> MAKDIEISASESKFILEALRQNYRLDGRSFDQFRDVEITFGKEFGDVSVKMGNTKVHCRISCQIAQPYEDRPFEGLFVISTEISPMAGSQFENGNITGEDEVLCSRIIEKSVRRSGALDVEGLCIVAGSKCWAVRADVHFLDCDGGFIDASCIAVMAGLMHFKKPDITVHGEQIIVHPVNEREPVPLGILHIPICVTFSFFNPQDTEENIKGETNSEISIIDATLKEELLRDGVLTVTLNKNREVVQVSKAGGLPMDALTLMKCCHEAYSIIEKITDQILQLLKEDSEKRNKYAAMLTSENAREI;> GPDHMSRLEIYSPEGLRLDGRRWNELRRFESSINTHPHAADGSSYMEQGNNKIITLVKGPKEPRLKSQMDTSKALLNVSVNITKFSKFERSKSSHKNERRVLEIQTSLVRMFEKNVMLNIYPRTVIDIEIHVLEQDGGIMGSLINGITLALIDAGISMFDYISGISVGLYDTTPLLDTNSLEENAMSTVTLGVVGKSEKLSLLLVEDKIPLDRLENVLAIGIAGAHRVRDLMDEELRKHAQKRVSNASAR;> MAESTTLETIEIHPITFPPEVLARISPELSLQRHLSLGIRPCLRKYEEFRDVAIENNTLSRYADAGNIDTKNNILGSNVLKSGKTIVITSITGGIIEETSAAIKDLDDFGEEELFEVTKEEDIIANYASVYPVVEVERGRVGACTDEEMTISQKLHDSILHSRILPKKALKVKAGVRSANEDGTFSVLYPDELEDDTLNETNLKMKRKWSYVLYAKIVVLSRTGPVFDLCWNSLMYALQSVKLPRAFIDERASDLRMTIRTRGRSATIRETYEIICDQTKSVPLMINAKNIAFASNYGIVELDPECQLQNSDNSEEEEVDIDMDKLNTVLIADLDTEAEETSIHSTISILAAPSGNYKQLTLVGGGAKITPEMIKRSLLLSRVRADDLSTRFNI;> GSMSVQAEIGILDHVDGSSEFVSQDTKVICSVTGPIEPKARQELPTQLALEIIVRPAKGVATTREKVLEDKLRAVLTPLITRHCYPRQLCQITCQILESGEDEAEFSLRELSCCINAAFLALVDAGIALNSMCASIPIAIIKDTSDIIVDPTAEQLKISLSVHTLALEFVNGGKVVKNVLLLDSNGDFNEDQLFSLLELGEQKCQELVTNIRRIIQDNISPRLVV;> GDPHMSLSVAEKSYLYDSLASTPSIRPDGRLPHQFRPIEIFTDFLPSSNGSSRIIASDGSECIVSIKSKVVDHHVENELLQVDVDIAGQRDDALVVETITSLLNKVLKSGSGVDSSKLQLTKKYSFKIFVDVLVISSHSHPVSLISFAIYSALNSTYLPKLISAFDDLEVEELPTFHDYDMVKLDINPPLVFILAVVGNNMLLDPAANESEVANNGLIISWSNGKITSPIRSVALNDSNVKSFKPHLLKQGLAMVEKYAPDVVRSLENL;> MNVQDRRRLLGPAAAKPMAFSNTTTHVPEKKSTDLTPKGNESEQELSLHTGFIENCNGSALVEARSLGHQTSLITAVYGPRSIRGSFTSQGTISIQLKNGLLEKYNTNELKEVSSFLMGIFNSVVNLSRYPKSGIDIFVYLTYDKDLTNNPQDDDSQSKMMSSQISSLIPHCITSITLALADAGIELVDMAGAGEANGTVVSFIKNGEEIVGFWKDDGDDEDLLECLDRCKEQYNRYRDLMISCLMNQET;> GDPHMSTFIFPGDSFPVDPTTPVKLGPGIYCDPNTQEIRPVNTGVLHVSAKGKSGVQTAYIDYSSKRYIPSVNDFVIGVIIGTFSDSYKVSLQNFSSSVSLSYMAFPNASKKNRPTLQVGDLVYARVCTAEKELEAEIECFDSTTGRDAGFGILEDGMIIDVNLNFARQLLFNNDFPLLKVLAAHTKFEVAIGLNGKIWVKCEELSNTLACYRTIMECCQKNDTAAFKDIAKRQFKEILTVKEE;> GDPHMSEVITITKRNGAFQNSSNLSYNNTGISDDENDEEDIYMHDVNSASKSESDSQIVTPGELVTDDPIWMRGHGTYFLDNMTYSSVAGTVSRVNRLLSVIPLKGRYAPETGDHVVGRIAEVGNKRWKVDIGGKQHAVLMLGSVNLPGGILRRKSESDELQMRSFLKEGDLLNAEVQSLFQDGSASLHTRSLKYGKLRNGMFCQVPSSLIVRAKNHTHNLPGNITVVLGVNGYIWLRKTSQMDLARDTPSANNSSSIKSTGPTGAVSLNPSITRLEEESSWQIYSDENDPSISNNIRQAICRYANVIKALAFCEIGITQQRIVSAYEASMVYSNVGELIEKNVMESIGSDILTAEKMRGNGN;> GDPHMACNFQFPEIAYPGKLICPQYGTENKDGEDIIFNYVPGPGTKLIQYEHNGRTLEAITATLVGTVRCEEEKKTDQEEEREGTDQSTEEEKSVDASPNDVTRRTVKNILVSVLPGTEKGRKTNKYANNDFANNLPKEGDIVLTRVTRLSLQRANVEILAVEDKPSPIDSGIGSNGSGIVAAGGGSGAATFSVSQASSDLGETFRGIIRSQDVRSTDRDRVKVIECFKPGDIVRAQVLSLGDGTNYYLTTARNDLGVVFARAANGAGGLMYATDWQMMTSPVTGATEKRKCAKPF;> SLMVEKPQLKFKSPIDNSESHPFIPLLKEKPNALKPLSESLRLVDDDENNPSHYPHPYEYEIDHQEYSPEILQIREEIPSKSWDDSVPIWVDTSTELESMLEDLKNTKEIAVNLEHHDYRSYYGIVCLMQISTRERDYLVDTLKLRENLHILNEVFTNPSIVKVFHGAFMDIIWLQRDLGLYVVGLFDTYHASKAIGLPRHSLAYLLENFANFKTSKKYQLADWRIRPLSKPMTAYARADTHFLLNIYDQLRNKLIESNKLAGVLYESRNVAKRRFEYSKYRPLTPSSEVYSPIEKESPWKILMYQYNIPPEREVLVRELYQWRDLIARRDDESPRFVMPNQLLAALVAYTPTDVIGVVSLTNGVTEHVRQNAKLLANLIRDALRNIKNTNEEATPIPSSETKADGILLETISVPQIRDVMERFSVLCNSNISKSRAKPVTNSSILLGKILPREEHDIAYSKDGLPNKVKTEDIRIRAQNFKSALANLEDIIFEIEKPLVVPVKLEEIKTVDPASAPNHSPEIDNLDDLVVLKKKNIQKKQPAKEKGVTEKDAVDYSKI;> SLMSVPAIAPRRKRLADGLSVTQKVFVRSRNGGATKIVREHYLRSDIPCLSRSCTKCPQIVVPDAQNELPKFILSDSPLELSAPIGKHYVVLDTNVVLQAIDLLENPNCFFDVIVPQIVLDEVRNKSYPVYTRLRTLCRDSDDHKRFIVFHNEFSEHTFVERLPNETINDRNNRAIRKTCQWYSEHLKPYDINVVLVTNDRLNREAATKEVESNIITKSLVQYIELLPNADDIRDSIPQMDSFDKDLERDTFSDFTFPEYYSTARVMGGLKNGVLYQGNIQISEYNFLEGSVSLPRFSKPVLIVGQKNLNRAFNGDQVIVELLPQSEWKAPSSIVLDSEHFDVNDNPDIEAGDDDDNNESSSNTTVISDKQRRLLAKDAMIAQRSKKIQPTAKVVYIQRRSWRQYVGQLAPSSVDPQSSSTQNVFVILMDKCLPKVRIRTRRAAELLDKRIVISIDSWPTTHKYPLGHFVRDLGTIESAQAETEALLLEHDVEYRPFSKKVLECLPAEGHDWKAPTKLDDPEAVSKDPLLTKRKDLRDKLICSIDPPGCVDINDALHAKKLPNGNWEVGVHIADVTHFVKPGTALDAEGAARGTSVYLVDKRIDMLPMLLGTDLCSLKPYVDRFAFSVIWELDDSANIVNVNFMKSVIRSREAFSYEQAQLRIDDKTQNDELTMGMRALLKLSVKLKQKRLEAGALNLASPEVKVHMDSETSDPNEVEIKKLLATNSLVEEFMLLANISVARKIYDAFPQTAMLRRHAAPPSTNFEILNEMLNTRKNMSISLESSKALADSLDRCVDPEDPYFNTLVRIMSTRCMMAAQYFYSGAYSYPDFRHYGLAVDIYTHFTSPIRRYCDVVAHRQLAGAIGYEPLSLTHRDKNKMDMICRNINRKHRNAQFAGRASIEYYVGQVMRNNESTETGYVIKVFNNGIVVLVPKFGVEGLIRLDNLTEDPNSAAFDEVEYKLTFVPTNSDKPRDVYVFDKVEVQVRSVMDPITSKRKAELLLK;> GSVKRVVYKKRPNLIISNVGYSELRKPEGVISGRKTFGDNSD

The eukaryotic RNA exosome is a conserved and essential multisubunit complex that carries out diverse functions in RNA metabolism, ranging from normal turnover, processing and maturation, to quality control. In yeast, its 9-subunit core (Exo9) forms a donut-shaped scaffold that recruits two 3’ to 5’ exoribonucleases, Dis3 (aka Rrp44) and Rrp6. Subunit composition of RNA exosomes varies according to cellular localization, where Exo9 and Dis3 form the cytoplasmic exosome (Exo10Dis3), and Exo9, Dis3, and Rrp6 constitute the nuclear exosome (Exo11Dis3/Rrp6). The nuclear exosome is associated with the protein cofactors Mpp6 and Rrp47, whose individual deletion in vivo results in misprocessing of nuclear exosome substrates, while concomitant loss leads to synthetic lethality.

The crystal structure of Exo12Dis3exo-endo-/Rrp6exo-/Mpp6Min was determined to a resolution of 3.3 Å using a synthetic RNA with two 3’ ends. Analogous to the previous structure, one RNA 3’ end is anchored in the Dis3 active site with Dis3 adopting a ‘direct access’ conformation while the other 3’ end is anchored in the Rrp6 active site of an adjacent complex. Mpp6Minimal interacts with an extended surface across the S1/KH subunit, Rrp40. Electron densities for Mpp6 residues 90 to 118 were evident on the surface of Rrp40. Mpp6Minimal residues 90–97 adopt a distorted parallel beta-strand configuration that complements the second beta-strand of the Rrp40 N-terminal domain (NTD) while residues 98–103 adopt a helical conformation that wedges between the Rrp40 NTD and S1 domain. Mpp6 residues 110–118 adopt an anti-parallel beta-strand conformation that complements the second beta-strand of the KH domain. Mpp6 residues Leu92, Ile93 and Ile94 reside in the first beta strand and are nestled into a hydrophobic surface of the Rrp40 NTD. The most prominent electron density observed for Mpp6 corresponds to Arg112 within the last beta strand. Arg112 projects into a pocket formed between the S1 and KH domains of Rrp40 and resides in one of two regions of Mpp6 previously identified as conserved from yeast to man. RNA binding activities likely contribute, however alignment of Exo12Dis3exo-endo-/Rrp6exo-/Mpp6Min with Exo11Dis3exo-endo-/Rrp6exo- reveals changes in the orientation of the Rrp6 catalytic module (CAT) relative to Exo9 with Rrp6 CAT tilted by 15 degrees to a more open configuration in the complex containing Mpp6.> MASIPSAAPSWRKMQIPRPLQRLFDYFPLRIYEPNELPERSQQLTSGDLPTLYVFSTDSDARLGLPSFNPGCLKWQTLLRLANLDFRILPSTNHSSPTGSLPFLLPPRTSPTASPAPIPASGLLSFARKNPWRPGKAADLDLGHLDADLPPRAQAYLALITHSLRNAWLCALYLDPTHDALLRRLYVDPASSSRAVRAALLHQLRRAAAEQVATASSGGGKIVSLAPVDSADGIDEEAVYRSARDALDALASLLRESETAWFFGTERPGSFDAALFSYTHLMVEYMSEEEDTESAKGRVSLGRMVKEAGNGELAEHRERMLGVAWPEWDGYRR;> MASSLGFGGSNAVDKVNATTTPGTVATPNSGPTKMLDEHILTPASISTLEVHG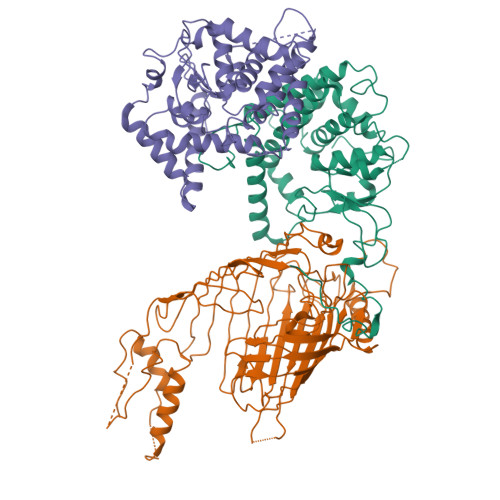ATNTRRSLLDQIFKPVLEDTAAAGTTLGQVLDRVGAATKKLARFDIFKEEGFGVFLSEAAPPQSAPPTDRTDLDISIRVKEKSRLVFSAGTDFGNAEGSAYTNAVVRNIFGGAETLTVNASTGTRTRSAYNATFSTPINGNPDLRLSVEALRSATQKPWASHEEHLTGANLRLAWLTEKGDTHALAYSSVWRQLTGLAPTASPTVRADAGDSLKSSLTHTFTRDRRDNPMLPQSGYLFRSVSELAGWGPLNGDVSFAKTEVEASGALPVAIPGLAGKSGVSVGGGLRLGVLYPLPLGYSLTGAAQPSRINDRFQLGGPNDVRGFKIGGLGPHDGVDAVGGDVFAAGSVNALLPLPRTGPDSPLRLQLYANAGRLVALNSKGTDKEGKEGLAMDSAAVFKGVKSAVGKLTNGIPSLAAGVGLVYAHPVARFELNFSLPLVLRRGEEGRKGLQVGVGISFL;> MAVQLHVWGPAFGLPSIDAECLAAIAYLAQTLGSADYQLIQSSPSAVPTQHLPTLYDSRTSTWIGGFTSITAHLHTHPPPTFQSAPQPTDGSSSTTTTTTTTTTAASATADGTAYTAFLSAHAAPLLALSLYVSSANYGAATRPAYSAVLPLPLPWTEPPAVRAAMARRAAHLGLSSLDADAAAERARAEERRAAADGWVAVPPHATAGRAAGGGGGGGGGGGKGGGVAAVLTPEQKSRIRLEEAAREVLDVLAEVDWAAGGGGRQVAAEVRCLAFGYLALMLLPDVPRPWLREIMEGRYPALCTFVRDFRARVFPQGGKLLPWADGGAQASASASASASAVALRFVRAVMAEVPLVGEWWSRWWTARKKREVLASKGAKPAPSNDLLLLLGAGLGLTVVGAGVFFYRGLPPFGEAVQVWRKPVVGLSSFGAAGAMFSGALYGLD4-(aminomethyl)benzene-1-sulfonamide | C7 H10 N2 O2 S | 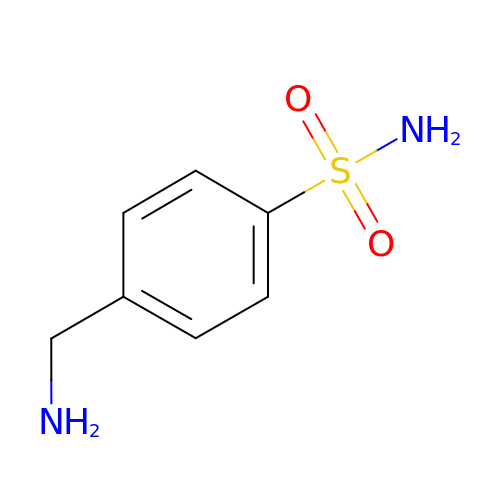TYMRLRRVMHJFTF-UHFFFAOYSA-N>[2x]GID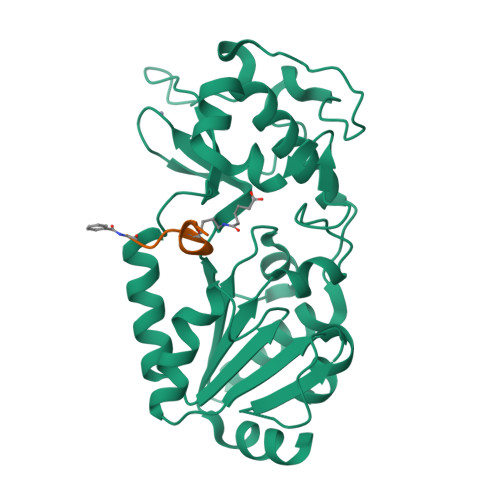PFTTRPSSDLTAFREHFAKAKHIAIITGAGVSAESGVPTFRGPGGFWRKWQAQDLATPEAFSRDPSLVWEFYHYRREVMRSKMPNPAHLAIAECEARLGQQGRSVVIITQNIDELHHRAGSKHVYEIHGSLFKTRCMSCGEVKANHKSPICPALDGKGAPDPNTKEARIPVELLPRCERKSCNGLLRPHVVWFGETLDSDILTAVERELEKCDLCLVVGTSSIVYPAAMFAPQVASRGVPVAEFNMECTPATQRFKYHFEGPCGSTLPPALE;> XGVLKEYGV Putidacin A (or LlpABW), first identified in Pseudomonas putida BW11M1, represents a class of Pseudomonas-specific antibacterial proteins not related to any known bacteriocin. The crystal structure of LlpABW from P. putida BW11M1 (LlpABW) shows it contains two β-prism MMBL domains, referred to as the N-domain and the C-domain following their position in the amino acid sequence. For the protein containing two similarly folded domains, we constructed site-specific mutants affected in carbohydrate binding and domain chimers from LlpA homologues to show that mannose-specific sugar binding mediated by one domain is required for activity and that the other domain determines target strain specificity. The LlpA branch occupies a unique position among MMBL-domain proteins, harboring non-eukaryotic representatives and being equipped with the capacity to kill bacterial cells with bacteriocin-like specificity, a property not yet demonstrated for other family members.

Soaks with oligomannoses revealed additional sugar-binding subsites. Binding site IIIC accommodates the disaccharide Manα(1–2)Man and the pentasaccharide GlcNAcβ(1–2)Manα(1–3)[GlcNAcβ(1–2)Manα(1–6)]Man. In the case of the pentasaccharide, the central reducing mannose is located in the shallow Me-Man binding site and the two GlcNAcβ(1–2)Man moieties stretch out over the surface making only a few additional hydrogen bonds or van der Waals contacts. Far UV CD spectra of these mutant forms are identical to that of native protein LlpABW, indicating that the mutations do not affect the overall structure of the protein. Isothermal titration calorimetry (ITC) showed that LlpABW has an affinity of 2.1 mM for the pentasaccharide GlcNAcβ(1–2)Manα(1–3)[GlcNAcβ(1–2)Manα(1–6)]Man, the highest among all the tested oligo-mannosides (See Figure 5 and Table 1 for a summary of the experimentally validated LlpABW-carbohydrate interactions).

>MAGRTRIPFNGVGTSVLPAYQTLSAGQYLLSPNQRFKLLLQGDGNLVIQDNGATVWVANEQQPFSSTIPLRNKKAPLAFYVQYGAFLDDYSRRRVWLTDNSTFTSNDQWNRTHLVLQDDGNIVLVDSLALWNGTPAIPLVPGAIDSLLLAPGSELVQGVVYGAGASKLVFQGDGNLVAYGPNGAATWNAGTQGKGAVRAVFQGDGNLVVYGAGNAVLWHSHTGGHASAVLRLQANGSIAILDEKPVWARFGFQPTYRHIRKINPDQKPIDIWTWHF[2x]>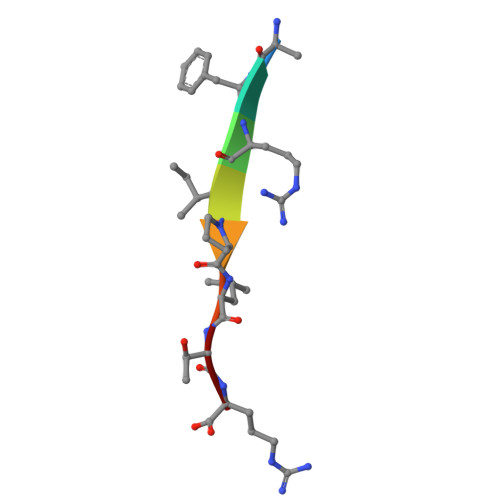 AFRIPLTR> MLDNVLRIATRQ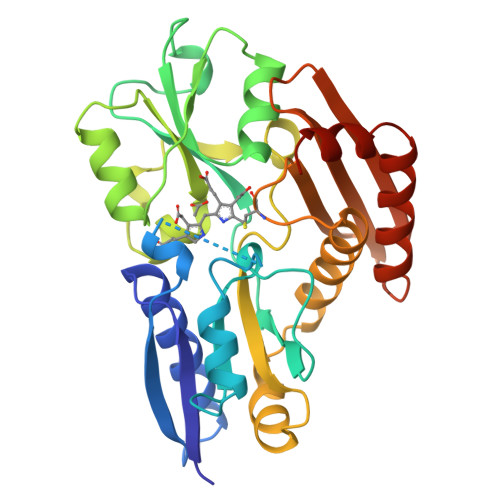SPLALWQAHYVKDKLMASHPGLVVELVPMVTRGDVILDTPLAKVGGKGLFVKELEVALLENRADIAVHSMKDVPVEFPQGLGLVTICEREDPRDAFVSNNYDSLDALPAGSIVGTSSLRRQCQLAERRPDLIIRSLRGNVGTRLSKLDNGEYDAIILAVAGLKRLGLESRIRAALPPEISLPAVGQGAVGIECRLDDSRTRELLAALNHHETALRVTAERAMNTRLEGACQVPIGSYAELIDGEIWLRGLVGAPDGSQIIRGERRGAPQDAEQMGISLAEELLNNGAREILAEVYNGDAPA> TGAITVGNKNNDKLTLWTTPAPSPNCRLNAEKDAKLTLVLTKCGSQILATVSVLAVK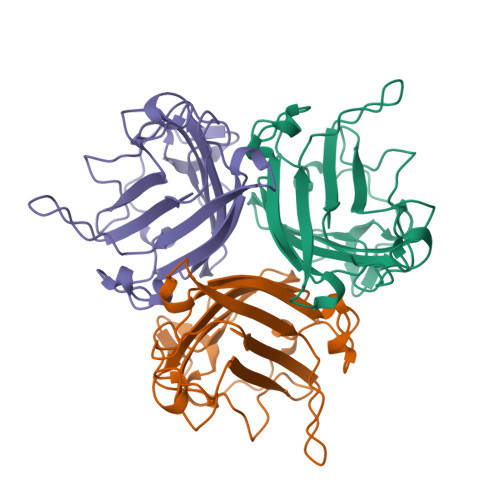GSLAPISGTVQSAHLIIRFDENGVLLNNSFLDPEYWNFRNGDLTEGTAYTNAVGFMPNLSAYPKSHGKTAKSNIVSQVYLNGDKTKPVTLTITLNGTQETGDTTPSAYSMSFSWDWSGHNYINEIFATSSYTFSYIAQE> SAPADYFRILVQQFEVQLQQYRQQIEELENHLATQANNSHITPQDLSMAMQKIYQT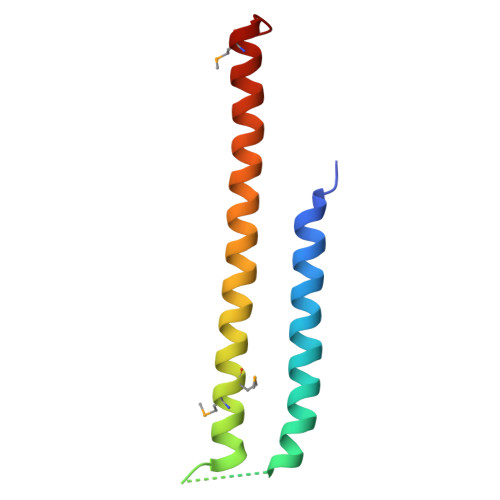FVALAAQLQSIHENVKVLKEQYLGYRKMFLGDA> ADYDLKFGMNAGT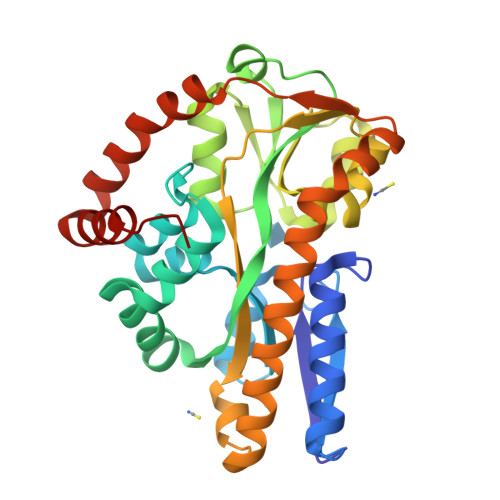SSNEYKAAEMFAKEVKEKSQGKIEISLYPSSQLGDDRAMLKQLKDGSLDFTFAESARFQLFYPEAAVFALPYVISNYNVAQKALFDTEFGKDLIKKMDKDLGVTLLSQAYNGTRQTTSNRAINSIADMKGLKLRVPNAATNLAYAKYVGASPTPMAFSEVYLALQTNAVDGQENPLAAVQAQKFYEVQKFLAMTNHILNDQLYLVSNETYKELPEDLQKVVKDAAENAAKYHTKLFVDGEKDLVTFFEKQGVKITHPDLVPFKESMKPYYAEFVKQTGQKGESALKQIEAINPHH> GSRRASVGSMARPAFVNKLWSMVNDKSNEKFIHWSTSGESIVVPNRERFVQEVLPKYFKHSNFASFVRQLNM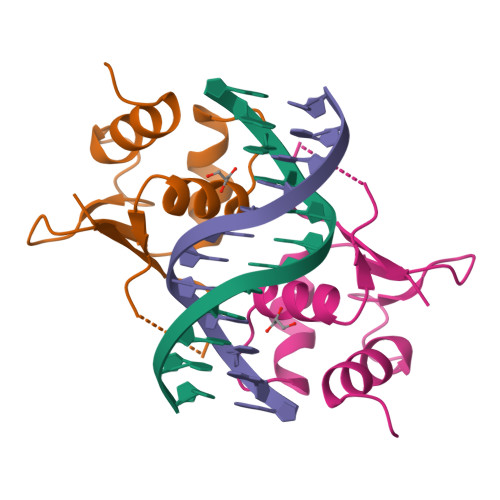YGWHKVQDVKSGSMLSNNDSRWEFENERHA>[2x]AKPDRSSFVPSLFSKKKKNVTMRSIKTTRDRVPTYQYNMNFEKLGKCIIINNKNFDKVTGMGVRNGTDKDAEALFKCFRSLGFDVI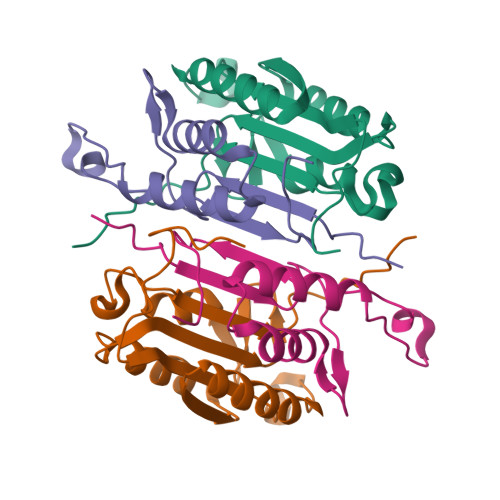VYNDCSCAKMQDLLKKASEEDHTNAACFACILLSHGEENVIYGKDGVTPIKDLTAHFRGDRCKTLLEKPKLFFIQACRGTELDDGIQ;>ANPRYKIPVEADFLFAYSTVPGYYSWRSPGRGSWFVQALCSILEEHGKDLEIMQILTRVNDRVARHFESQSDDPHFHEKKQIPCVVSMLTKELYFSQ[2x]> GEKGTTGTGNAALDNIFERKSVRTYLNKGVEKEKIDLMLRAGMSAPSGK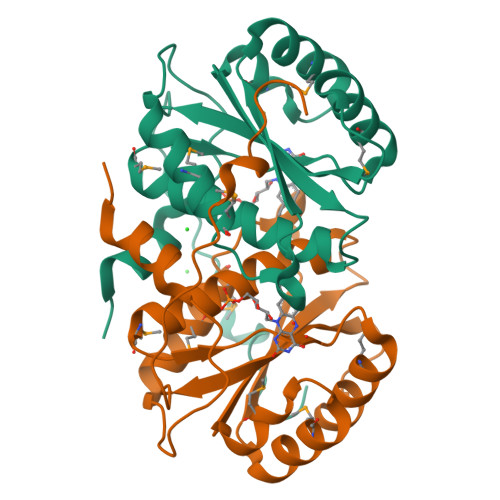DVRPWEFVVVSDRAKLDSMAAALPYAKMLTQARNAIIVCGDSARSFYWYLDCSAAAQNILLAAESMGLGAVWTAAYPYEDRMEVVRKYTHLPENILPLCVIPFGYPATKEQPKQKYDEKKIHYNQY> RGSHRILNLVKYDLYSIFKSPLTYLAILVVSSLIATQSILMANSMDNPKHIIVYGSVFAAAKWLLLIIGLMFVVKTITRD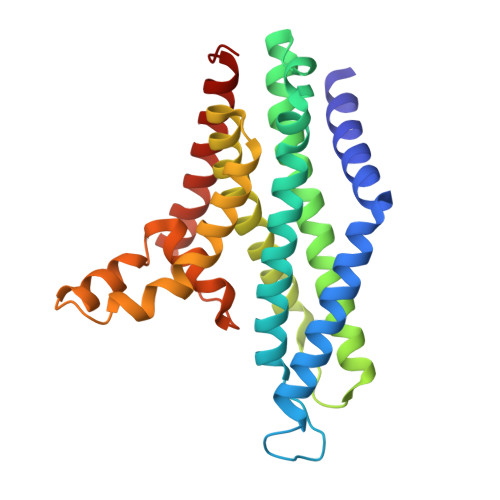FSQGTIQLYMSKVKTRVGYIISKTISIILISILFALIHYVILIVVQASSNGKNLAFSKYVDNLWFFLIFLLFFGLFLFLITLASQKTAMIFSLGVFLVLIVPFIKPFITFIPRYGEKVLDAFDYIPFAYLTDKMISSNFDFSNWQWVISLGSIVIFFILNILYVAKKDI>[2x]MNHKVHHHHHHIEGRHMYSPDRR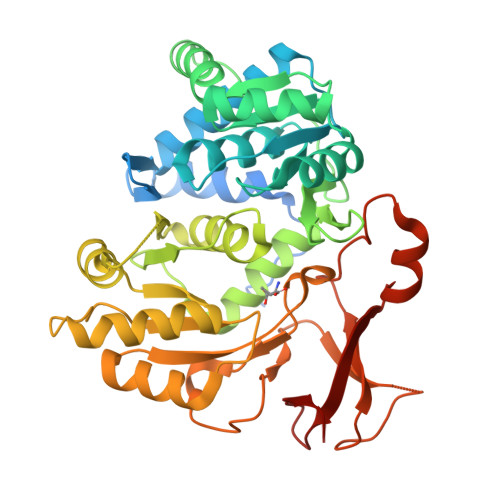AALNSVANMVSDNADKDLRYGGLVHDLLADSGKATPNSDAMEDAFGTWTYQELLNHSQAFSAWLDGKGVARGERIVVQLPNIRQTVAVFYGACRRGVVFVPLNPGMKPFHLRSVIADADPRLVIAEDETAADRLRDVTDLPVYSIDSLWADVERLRDAGAGAEAVEVSPEDLAVLIYTSGSTAAPKAVACPHQQIVFAASSINAVLGYHAEDIVFCRMSVSWDFGLYKVLISTLTGAKLVLAGGEPDIALVKSLRESGATMMPIVPSLASMLTTLIRRDPEGAPTLRMFTNSAAALPQVTIDALRSAFPGAQVVRMYGQTECKRISIMPPHLEHERPDSVGLPLPGTTIEILDEDGTLLPPGEPGEITVTGPHVMAGYWRAPEITARAYRRDETTGAMRLHTGDYGHLDEDGFLYFGGR Nek2 (NIMA-related kinase 2) is a human cell cycle-dependent serine/threonine protein kinase that localizes to the centrosome. However, Nek2 does play a key role in ensuring timely assembly of the mitotic spindle, a scaffold that is vital for accurate segregation of sister chromatids during mitosis. Phosphorylation of these proteins by Nek2 in late G2 promotes linker disassembly and loss of centrosome cohesion; this in turn allows the timely separation of centrosomes in prophase.

Preliminary data attained following a medium-throughput screening campaign, identified purines bearing 6-alkoxy substituents (e.g. 6; CDK2 IC50 = 0.005 μM; Nek2 IC50 = 12 μM) as dual inhibitors of Nek2 and CDK2. Interestingly, deletion of the sulfonamide moiety from 6, resulted in a 200-fold reduction in CDK2 inhibitor activity as well as some reduction in Nek2 activity (2-aminophenyl-6-(cyclohexylmethoxy)-9H-purine: CDK2 IC50 = 1 μM; Nek2 IC50 = 22 μM).

> MPSRAEDYEVLYTIGTGSYGRCQKIRRKSDGKILVWKELDYGSMTEAEKQMLVSEVNLLRELKHPNIVRYYDRIIDRTNTTLYIVMEYCEGGDLASVITKGTKERQYLDEEFVLRVMTQLTLALKECHRRSDGGHTVLHRDLKPANVFLDGKQNVKLGDFGLARILNHDTSFAKAFVGTPYYMSPEQMNRMSYNEKSDIWSLGCLLYELCALMPPFTAFSQKELAGKIREGKFRRIPYRYSDELNEIITRMLNLKDYHRPSVEEILENPLILEHHHHHH>SVRDELVWIDCEMTGLDLKSDRLIEIAVLVTDADLNILGDGLDVVIHADDESLSSMVDVVKQMHARSGLTEEVRRSTVDLATAEEMVLDYIRGHVKQAKTAPLAGNSIATDRGFIARDMPKLDDYLHYRMIDVSSIKELCRRWYPRIYFGQ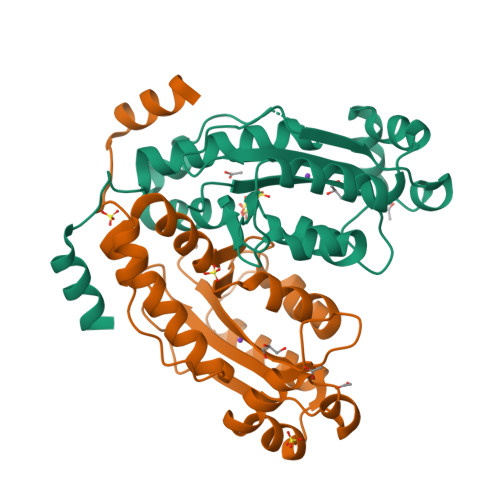PEKGLAHRALADIHESIRELKYYRATAFVPQPGPSTSDIAAIAAELGPPSSNSADTDSA[4x]> GPGSAESPKSTETSANGADKLADAYNTLLTEHEKLRDEYYTLIDAKEEEPRYKALRGENQD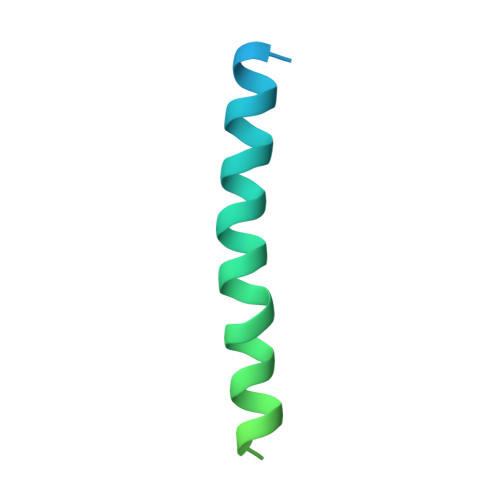LREKEGKYQDKIKKLEEKEKNLEKKSEDVERHYLKKLDQEHKE>MCAQPTASTVEGLFKPSSAFADRTDFSLSSILQKSLINRESFNQYLAMRLAPVLRTFYEDNYDTDIKERLNGFTADTDNAFVSQEQNLRNQFRENYLVHLQTDIFDNTGGNQAAWKLRDVNNKIIDDFISRIFAKNFVEYVQDGVGPLTKPTKSLIENTSNFKNIKLQPKFVNKNAKLKINNDAVYAAIQDKLLDQFITNENPNLVSRVVFTNETPVDGFDNYFNTKVIQSPTPSYQFQVFNKYNQQSGGTKGANGFNLLASNLKSYKNDQSKGIDIPNKFSSDSGGKLLLKASDMFDTFDPSFSAAFIQGYLALQKKSKGADSKEVDSLIKDKSIIENFFVDNNTQAAAAARAASSSSEGTIQLKTASDGGGTTQSTVHKTDLVKIFGDKDVFAGEYKQQIGNTNANQTGGGGSGGGGG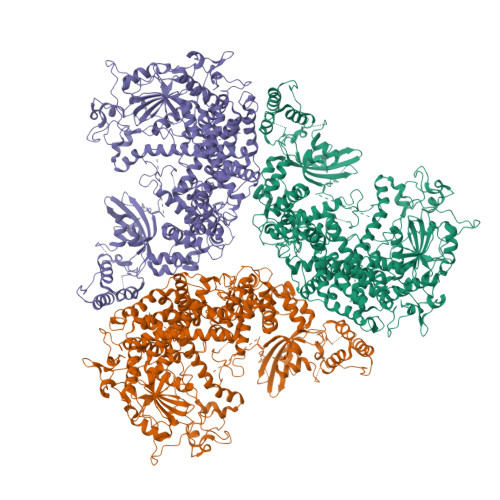TSTGSSTGSSTETTTGNSSKAVVDLIEVKKDSSSQPDYILSRGKDGIHLMAVDGGSHYLTESGRDVAKQKKFLLFRALQTKYGLVDTDTTYDFKLFDEVKKYFDTNRILFLFEALLDLSSDTNNKDNFLSYPQFKKFADSIKSIEKDLKELVQAHYKQAVFNETAVAENKVTLKLAERNQPFIDNERNNQIEQNGLAAKLPYEQDAKTGHYNDLGNYYKDIIDNVDKKGTSTVKTTSSNTGQTKNFSEEVVSKLKDNKKKVEEAAKKHVEALKVFTIPSPLYSQVILVQTKLSFTPESTSLGLNLALNNYLTSTELQNSIKLSYFQEDEAFKKIIDITNLTFSQQSGGTGGTNGNNNLTADNWKIFKETYLLDLFESQAQKSIFGHVGSSDKNSSTKTGIEGVLDTLYSSLNLEERLDSDDVIDYLSYLYTAHWLLKDNLKNYKQSLQSKLSRTSNAFLVWSVDSEKNKNDSQSTLSSTASSTSNTGLIQLRSVVSLAQNQAAGQGGDNNSDITQTEVKNPNFVFGSSVYDWTNSKTPEVNRAADDTSSFFYTKSSSSSTGAAQSSATVLRSLNQASGMTTKTAKNRYGFRGIVTSSTSGSLPEAVSRRLFKQFVNQTEKGVKVGGQMLITTAKSGKATLVLKQQADDAESTTNNAYKGALFSFGSMDNLKNIINGIQTQTEFDALYNHLTSDLNIDVTGVDKNKTLTEQKTSLTSFVDSNFKQSTQSAQRGDTSARSARSATVQIKKTQEDNQNTNYKDVFSRFDGYIGDNKVEEKNYTSYQFLSDGGKYHATFVKQVNLDDVEKIGTDSLKQEDSSKDKRLNLSLEEFLAAIALEALDPNNQTQAINALISGNKKGLVKVGDFRIFSSISAQWVRRFAAALEHHHHHH[3x]> MTPGKLYTLRYEVEGGGFIEIATVRPETVFADQAIAVHPEDERYRHLLGKRAR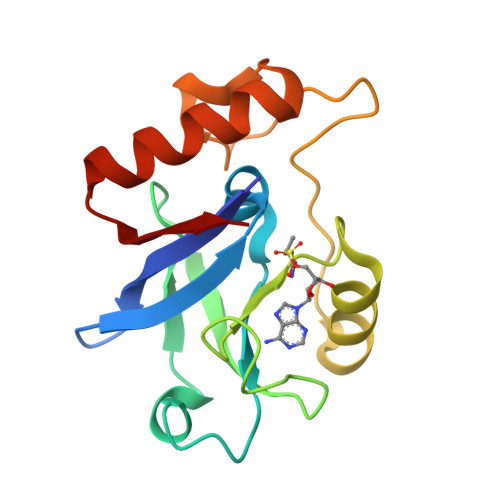IPLTEVWIPILADPAVEKDFGTGALKVTPAHDPLDYEIGERHGLKPVSVINLEGRMEGERVPEALRGLDRFEARRKAVELFREAGHLVKEEDY>GUGUGU[2x]

Poly(UG) or ‘pUG’ dinucleotide repeats are highly abundant sequences in eukaryotic RNAs. In Caenorhabditis elegans, pUGs are added to RNA 3′ ends to direct gene silencing within Mutator foci, a germ granule condensate. Here, we show that pUG RNAs efficiently self-assemble into gel condensates through quadruplex (G4) interactions. Short pUG sequences form right-handed intermolecular G4s (pUG G4s), while longer pUGs form left-handed intramolecular G4s (pUG folds).

We determined the structure of the (GU)3 pUG G4 by single crystal x-ray diffraction methods to a maximum resolution of 1.05 Å. The structure contains eight hexanucleotide strands (48 nucleotides) and forms a dimer of right-handed parallel quadruplexes. The dimer is a 5′–5′ head-to-head stack of G4s mediated through a shared potassium ion coordinated between the first quartets. A total of seven potassium ions are coordinated between the quartets, and eight sodium ions are bound at the 3′ ends. The structure contains six G-quartets, four U-quartets and eight bulged uridines. The right-handed parallel pUG G4 forms a continuous stack of G and U quartets except for the U2 nucleotides which bulge out and stack on each other. The two stacked pUG G4s are in different conformations, hereafter referred to as A and B (pUG G4A and pUG G4B). There are no ions between the G3 and U4 quartets, and only in pUG G4B is there is a single buried water molecule at this location. The water binding site is created by the closer stacking of the G3B and U4B quartets (3.4 Å versus 3.9 Å for G3A and U4A). On the other hand, the G3B sugar puckers sample the C2′ and C3′ endo conformations almost equally. These data suggest the buried water molecule helps to stabilize the G3B C3′ endo conformation.Nanos is a conserved post-transcriptional mRNA regulator that was first identified as being required for posterior pattern formation in the Drosophila melanogaster embryo. Although the Nanos partners vary depending on the organism and mRNA target, a common emerging partner is the CCR4–NOT deadenylase complex, which interacts with the N-terminal region of Nanos proteins in diverse organisms. The CCR4–NOT deadenylase complex plays a central role in post-transcriptional mRNA regulation by catalyzing the removal of mRNA poly(A) tails, repressing translation, and promoting mRNA degradation. The CNOT1-C region contains the NOT1 superfamily homology domain (SHD), which interacts with CNOT2–CNOT3 heterodimers to form the NOT module.

To this end, we crystallized the CNOT1 SHD (residues 1833–2361) in complex with the NIM peptide of Nanos1 (residues 40–56). The CNOT1–Nanos1 crystals contain two molecules of CNOT1 sandwiching two Nanos1 peptides between them. The other Nanos1 peptide (chain B) contacts the helices of the final HEAT-like repeat of CNOT1 (chain A, α22 and α23). Because this helix arrangement is conserved in three independent NOT1 structures from three different organisms, it is unlikely to be the result of crystal contacts. In contrast, helix α23 displays two additional turns in the structure of the CNOT1–Nanos1 complex (Fig. 5G–I gray helix) and moves by 43° relative to its position in the human NOT module (salmon helix), which results in the opening up of the Nanos-binding site. The first eight residues of the Nanos1 peptide form a turn and a short α helix that lies almost perpendicular on top of the CNOT1 helix α23, thereby covering the hydrophobic pocket. More specifically, three highly conserved aromatic residues (namely, F40, W43, and Y46) insert deep inside the CNOT1 pocket, where Y46 forms a hydrogen bond with the backbone oxygen of CNOT1 F2353. The orientation of the turn is fixed by the invariant residue D45, which provides two intramolecular hydrogen bonds (one to the backbone amide nitrogen and one to the hydroxyl group of S41). The other invariant NIM residue, L49, is located at the end of the short helix. This residue makes hydrophobic contacts with A2357 of CNOT1 and packs against Nanos1 F40 and Y46, which most likely results in the stabilization of the overall conformation of the peptide.

>[2x]GPHMLEHSGISQASEYDDPPGLREKAEYLLREWVNLYHSAAAGRDSTKAFSAFVGQMHQQGILKTDDLITRFFRLCTEMCVEISYRAQAEQQHNPAANPTMIRAKCYHNLDAFVRLIALLVKHSGEATNTVTKINLLNKVLGIVVGVLLQDHDVRQSEFQQLPYHRIFIMLLLELNAPEHVLETINFQTLTAFCNTFHILRPTKAPGFVYAWLELISHRIFIARMLAHTPQQKGWPMYAQLLIDLFKYLAPFLRNVELTKPMQILYKGTLRVLLVLLHDFPEFLCDYHYGFCDVIPPNCIQLRNLILSAFPRNMRLPDPFTPNLKVDMLSEINIAPRILTNFTGVMPPQFKKDLDSYLKTRSPVTFLSDLRSNLQVSNEPGNRYNLQLINALVLYVGTQAIAHIHNKGSTPSMSTITHSAHMDIFQNLAVDLDTEGRYLFLNAIANQLRYPNSHTHYFSCTMLYLFAEANTEAIQEQITRVLLERLIVNRPHPWGLLITFIELIKNPAFKFWNHEFVHCAPEIEKLFQSVAQCCM;>[2x]FSSWNDYLGLATLITKA>[3x]MSVEDTQPLITHLIELRKRLLNCIIAVIVIFLCLVYFAND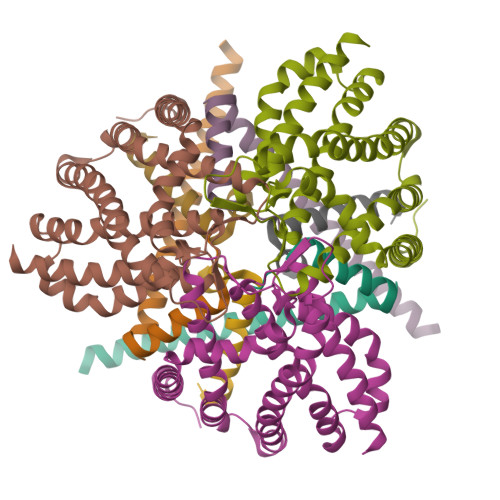IYHLVSAPLIKQLPQGSTMIATDVASPFFTPIKLTFMVSLILSAPVILYQVWAFIAPALYKHERRLVVPLLVSSSLLFYIGMAFAYFVVFPLAFGFLANTAPEGVQVSTDIASYLSFVMALFMAFGVSFEVPVAIVLLCWMGITSPEDLRKKRPYVLVGAFVVGMLLTPPDVFSQTLLAIPMYCLFEIGVFFSRFYVGKGRNREEENDAEAESEKTEERSHHHHHH;>MFDIGFSELLLVFIIGLVVLGPQRLPVAVKTVAGWIRALRSLATTVQNELTQELKLQEFQDSLKKVEKASLTNLTPELKASMDELRQAAESMKRSYVANDPEKASDEAHTIHNPVVKDNEAAHEGVTPAAAQTQASSPEQKPETTPEPVVKPAADAEPKTAAPSPSSSDKP[3x];>[3x]SMDRRRFIKGSMAMAAVCGTSGIASLFSQAAFAADSDIADGQTQRFDFSILQSMAHDLAQTAWRGAPRPLPDTLATMTPQAYNSIQYDAEKSLWHNVENRQLDAQFFHMGMGFRRRVRMFSVDPATHLAREIHFRPELFKYNDAGVDTKQLEGQSDLGFAGFRVFKAPELARRDVVSFLGASYFRAVDDTYQYGLSARGLAIDTYTDSKEEFPDFTAFWFDTVKPGATTFTVYALLDSASITGAYKFTIHCEKSQVIMDVENHLYARKDIKQLGIAPMTSMFSCGTNERRMCDTIHPQIHDSDRLSMWRGNGEWICRPLNNPQKLQFNAYTDNNPKGFGLLQLDRDFSHYQDIMGWYNKRPSLWVEPRNKWGKGTIGLMEIPTTGETLDNIVCFWQPEKAVKAGDEFAFQYRLYWSAQPPVHCPLARVMATRTGMGGFSEGWAPGEHYPEKWARRFAVDFVGGDLKAAAPKGIEPVITLSSGEAKQIEILYIEPIDGYRIQFDWYPTSDSTDPVDMRMYLRCQGDAISETWLYQYFPPAPDKRQYVDDRVMS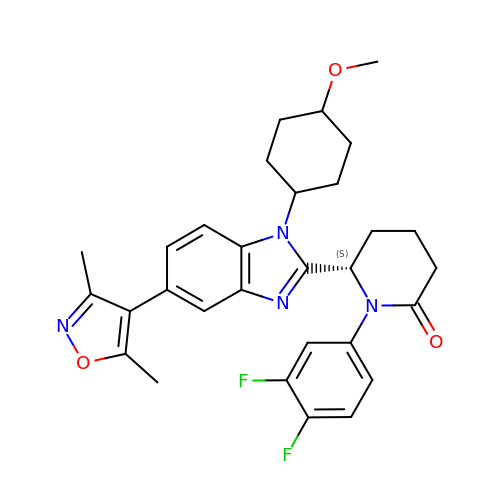(6S)-1-[3,4-bis(fluoranyl)phenyl]-6-[5-(3,5-dimethyl-1,2-oxazol-4-yl)-1-(4-methoxycyclohexyl)benzimidazol-2-yl]piperidin-2-one | C30 H32 F2 N4 O3 | SKDNDJWEBPQKCS-CLHVYKLBSA-N>[2x]ELTPDQQTLLHFIMDSYNKQRMPQEITNKILKEEFSAEENFLILTEMATNHVQVLVEFTKKLPGFQTLDHEDQIALLKGSAVEAMFLRSAEIF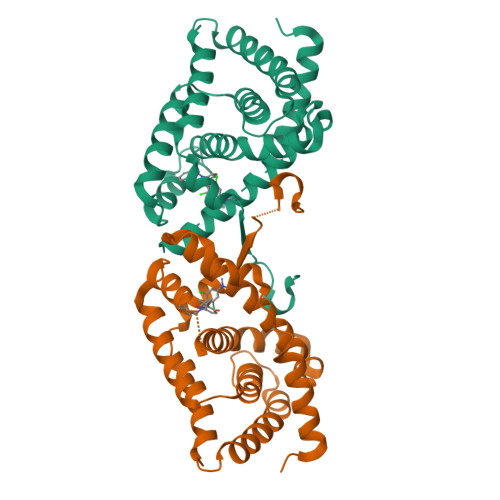NKKLPSGHSDLLEERIRNSGISDEYITPMFSFYKSIGELKMTQEEYALLTAIVILSPDRQYIKDREAVEKLQEPLLDVLQKLCKIHQPENPQHFAELLGRLTELRTFNHHHAEMLMSWRVNDHKFTPLLEEIW> MAIYADNSYSIGNTPLVRLKHFGHNGNVVVKIEGRNPSYSVKCRIGANMVWQAEKDGTLTKGKEIVDPTSGNTGIALAYVAAARGYKITLTMPETMSLERKRLLCGLGVNLVLTEGAKGMKGAIAKAEEIVASDPSRYVMLKQFENPANPQIHRETTGPEIWKDTDGKVDVVVAGVGTGGSITGISRAIKLDFGKQITSVAVEPVESPVISQTLAGEEVKPGPHKIQGIGAGFIPKNLDLSIIDRVETVDSDTALATARRLMAEEGILAGISSGAAV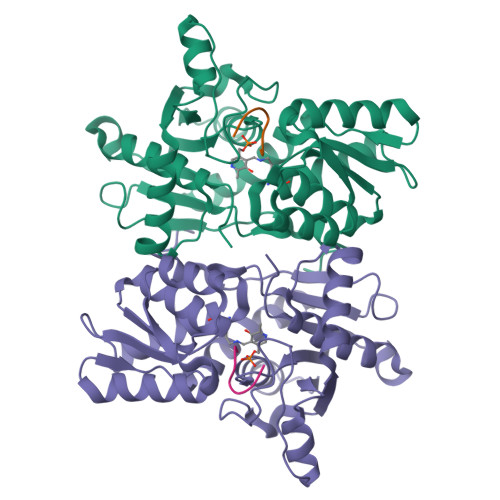AAADRLAKLPEFADKLIVVILPSASERYLSTALFEGIEG;> IGDGYEFT>[2x]MVISRAEIYWADLGPPSGSQPAKRRPVLVIQSDPYNASRLATVIA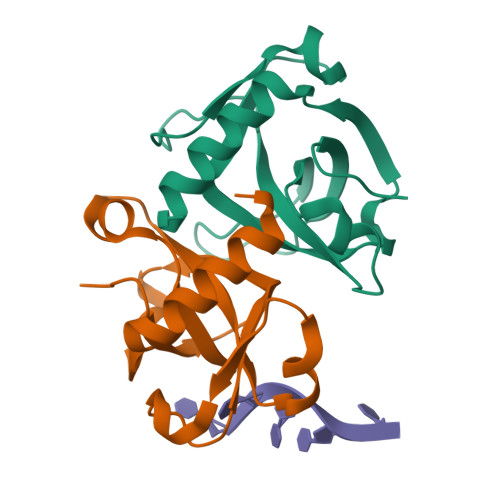AVITSNDALAAMPGNVDLPATTTRLPRDSVVNVTAIVTLNKTDLTDRVGEVPASLMHEVDRGLRRVLDL(2R,3S,4S,5R)-2-[2-(methylsulfanyl)ethyl]piperidine-3,4,5-triol | C8 H17 N O3 S 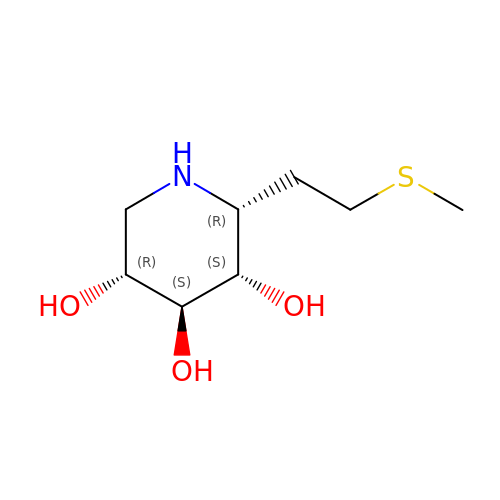| ZTGUKWHBLOJEPU-NGJRWZKOSA-N>[2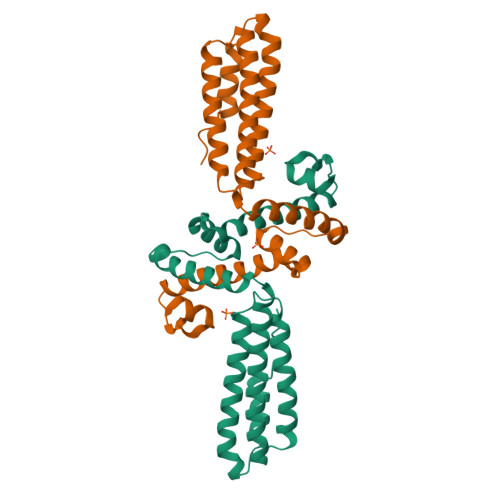x]GPLGSMKLRVENPKKAQKHFVQNLNNVVFTNKELEDIYNLSNKEETKEVLKLFKLKVNQFYRHAFGIVNDYNGLLEYKEIFNMMFLKLSVVFDTQRKEANNVEQIKRNIAILDEIMAKADNDLSYFISQNKNFQELWDKAVKLTKEMKIKLKGQKLDLRDGEVAINKVRELFGSDKNVKELWWFRSLLVKGVYLIKRYYEGDIELATTSDFAKAVFE>[2x]AMSLNIITVTLNMEKYNFLGISIVGQSNERGDG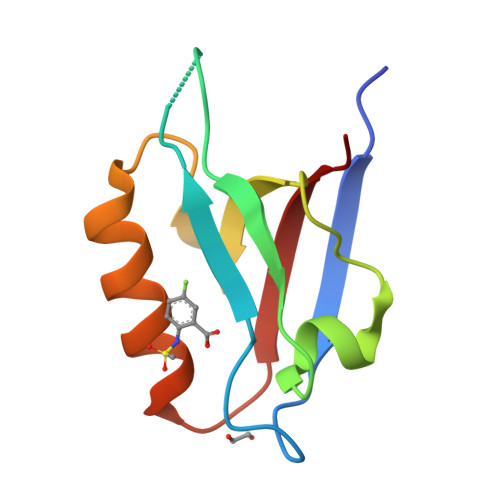GIYIGSIMKGGAVAADGRIEPGDMLLQVNEINFENMSNDDAVRVLREIVHKPGPITLTVAKS>GGKKFILELIETVYEEILDLEANLRNGQQTDSTAMWEALHIDDSSYD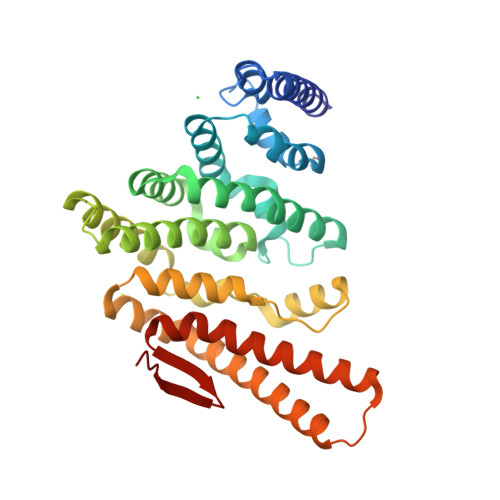VNPFISMLSFDKGIKIMPRIFNFLDKQQKLKILQKIFNELSHLQIIILSSYKTTPKPTLTQLKKVDLFQMIILKIIVSFLSNNSNFIEIMGLLLQLIRNNNVSFLTTSKIGLNLITILISRAALIKQDSSRSNILSSPEISTWNEIYDKLFTSLESKIQLIFPPREYNDHIMRLQNDKFMDEAYIWQFLASLALSGKLNHQRIIIDEVRDEIFATINEAETLQKKEKELSVLPQRSQELDTELKSIIYNKEKLYQDLNLFLNVMGLVYRDGEISELKHHHHHH[3x]> 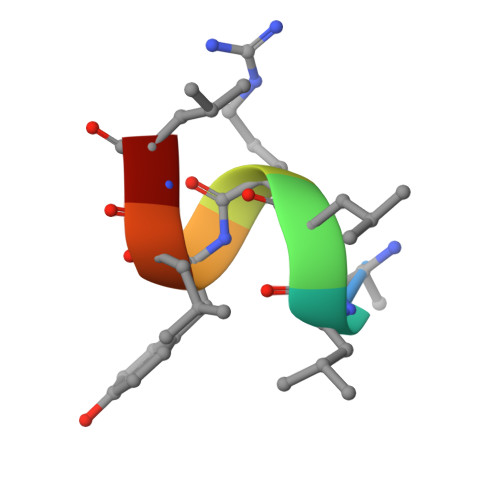ALLRYLLD>[2x]HMKERLLDELTLEGVARYMQSERCRRVICLVGAGISTSAGIPDFRSPSTGLYDNLEKYHLPYPEA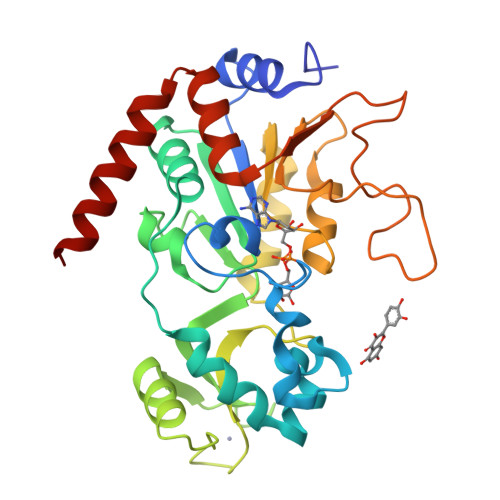IFEISYFKKHPEPFFALAKELYPGQFKPTICHYFMRLLKDKGLLLRCYTQNIDTLERIAGLEQEDLVEAHGTFYTSHCVSASCRHEYPLSWMKEKIFSEVTPKCEDCQSLVKPDIVFFGESLPARFFSCMQSDFLKVDLLLVMGTSLQVQPFASLISKAPLSTPRLLINKEKAGQSDPFLGMIMGLGGGMDFDSKKAYRDVAWLGECDQGCLALAELLGWKKELEDLVRREHASIDAQS>HHHHHHGS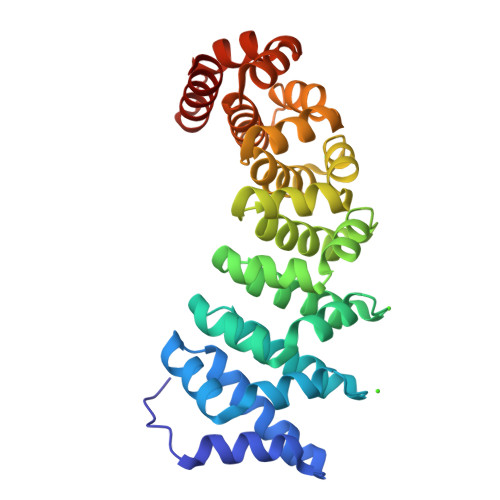ELPQMVQQLNSPDQQELQSALRKLSQIASGGNEQIQAVIDAGALPALVQLLSSPNEQILQEALWTLGNIASGGNEQIQAVIDAGALPALVQLLSSPNEQILQEALWTLGNIASGGNEQIQAVIDAGALPALVQLLSSPNEQILQEALWTLGNIASGGNEQIQAVIDAGALPALVQLLSSPNEQILQEALWTLGNIASGGNEQIQAVIDAGALPALVQLLSSPNEQILQEALWTLGNIASGGNEQKQAVKEAGALEKLEQLQSHENEKIQKEAQEALEKLQA[4x]> HMSQSNRELVVDFLSYKLSQKGYSWSQMAAVKQALREAGDEFELRYRRAFSDLTSQLHITPGTAYQSFEQVVNELFRDGVNWGRIVAFFSFGGALCVESVDKEMQVLVSRIAAWMATYLNDHLEPWIQENGGWDTFVELYG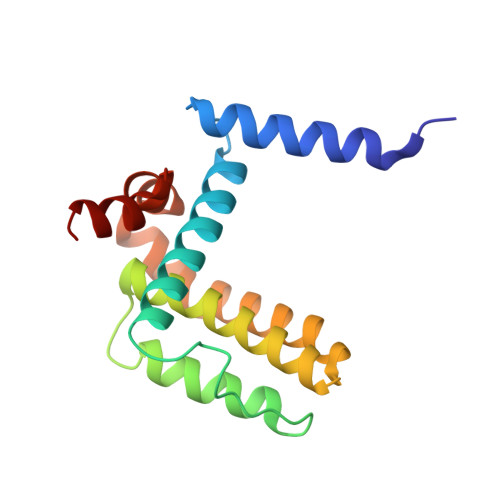NNAAAESRKGQE>AKGNDSKDFNNSYGISHITRDNMVKIPQQQNSDQFKVPAFDESTIKNIASAKGKNASGNTIDLDVWDSWPLQNADGTVATYHGYQIVFALAGDPKDSNDTSVYLFYKKAGDKSIDSWKNAGRVFKDSDKFVPNDPHLKNQTQEWSGSGTLTKDGKVRLFYTDYSGKQYGKQTLTTAQVNMSQPNDNTLKVDGVEDYKSIFDGDGKIYQTVQQFIDEGGADTGDNHTLRDPHYIEDNGHKYLVFEANTGTEDGYQGEDSLYNRAYYGGNNPFFQSEKKKLLEGSNKEKASLANGALGIIELNDDYTLKKVMKPLITSNTVTDEIERANIFKKDGKWYLFTDSRGSKMTIDGIGQDDVYMLGYVSNTLTGKYKPLNDTGLVLHMDLDPNDKTFTYSHFAVPQTKGDNVVITSYMTNRGFYEDNHSTFAPSFLVNIDGSKTSVVKDR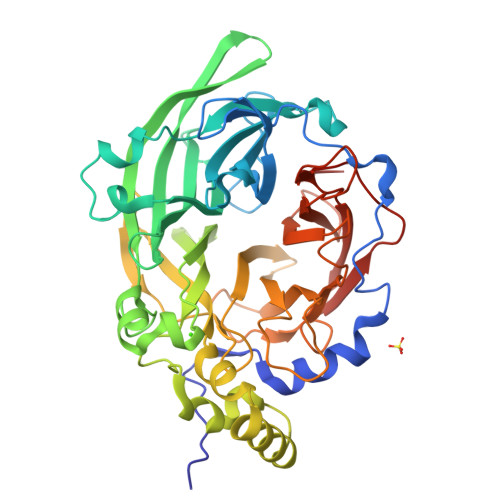VLEQGQLTVDED[4x]> GKELRQLQEDRKNDKKPPPYKHIKVNRPIGRVQIFTADLSEIPRCNCKATDENPCGIDSECINRMLLYECHPTVCPAGGRCQNQCFSKRQYPEVEIFRTLQRGWGLRTKTDIKKGEFVNEYVGELIDEEECRARIRYAQEHDITNFYMLTLDKDRIIDAGPKGNYARFMNHCCQPNCEAQK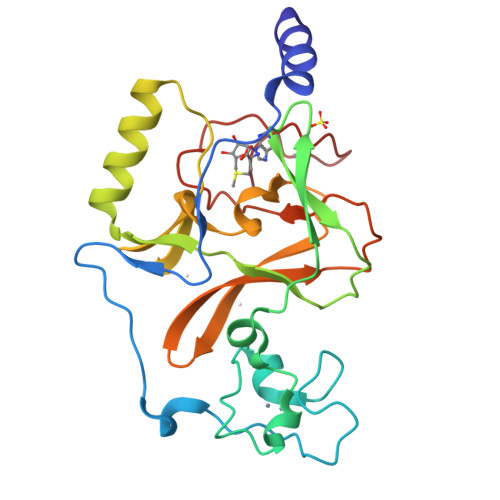WSVNGDTRVGLFALSDIKAGTELTFNYNLECLGNGKTVCKCGAPNCSGFLG> RGSHHHHHHGSFTPSGTTGTTKLTVTEECQVRVGDLTVAKTRGQLTDAAPIGPVTVQALGCNARQVALKADTDNFEQGKFFLISDNNRDKLYVN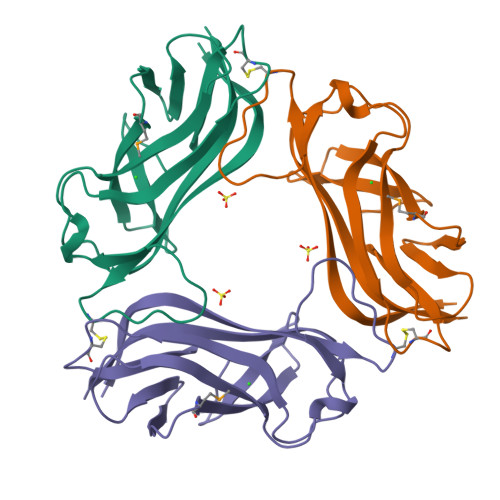IRPMDNSAWTTDNGVFYKNDVGSWGGTIGIYVDGQQTNTPPGNYTLTLTGGYWAK> SNAGGSSPITGLVYDQRMMLHHNMWDSHHPELPQRISRIFSRHEELRLLSRCHRIPARLATEEELALCHSSKHISIIKSSEHMKPRDLNRLGDEYNSIFISNESYTCALLAAGSCFNSAQAILTGQVRNAVAIVRPPGHHAEKDTACGFCFFNTAALTARYAQSITRESLRVLIVDWDVHHGNGTQHIFEEDDSVLYISLHRYEDGAFFPNSEDANY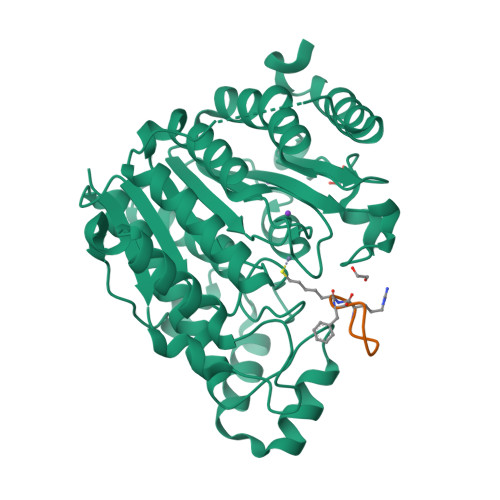DKVGLGKGRGYNVNIPWNGGKMGDPEYMAAFHHLVMPIAREFAPELVLVSAGFDAARGDPLGGFQVTPEGYAHLTHQLMSLAAGRVLIILEGGYNLTSISESMSMCTSMLLGDSPPSLDHLTPLKTSATVSINNVLRAHAPFWSSLR;> ASDRXFLK>GALRGGMTSQLNELVEFLHSPQPAVRQIAIDNLVGFSAGPTSKVFKNDSYRPIKDIIKMIMDPEHGTRVIIQQGVTILVNLSEDKLVRNIILSDDKKFLKFLVWKIVDLTNPNADIMCILLSNLAKDDGILAVLNIKRNSSGEEVDDGLKLAALNKEVFKSLRAMDCLMDCFVKGYDKKLTKYASFNYLAFFFADISRFKLGRMYFIEEQEYDGVVPISKLLVFTEKYDAKVRREGVASTIKNSLFDSETHERLLKDEKINLLPYILLPIASAK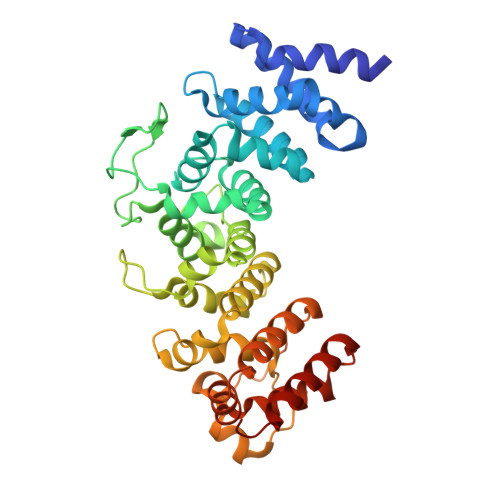DSEIDEEDMFNLPDELQLLPEDKERDPIPAIICCHLESILLLCTTHAGREYLRDKSVYPLVRELHKNVENEDIGELCYRIVNMLMRGEPGAGAVE[4x]> NLIDRGTYRKLPLFEGELPEGSYAQIVEVKPKQTVKKHYHERQYELFYIISGEAR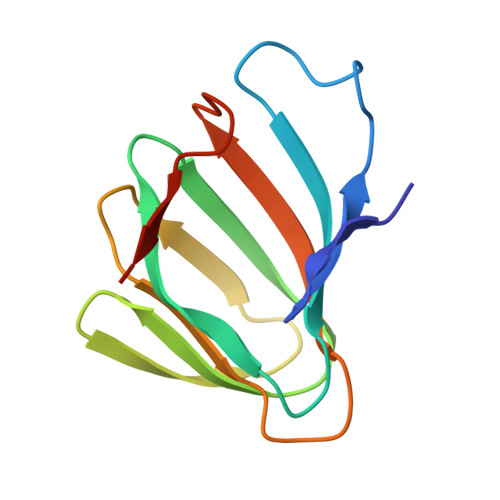LGIGDTEYQAKPGDIFLVKPKTVHWVVNEKDEPFRLFVVKLNYHGDDSVWLEGSF> GTQQK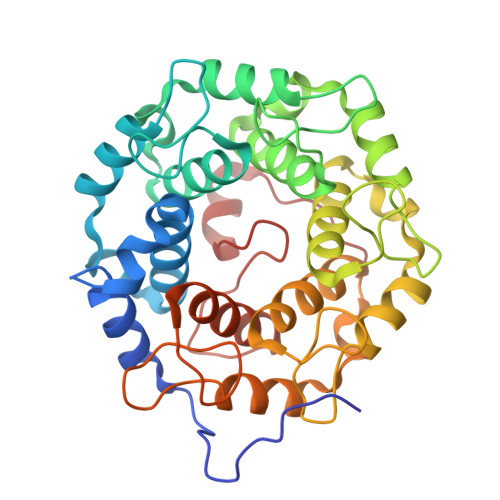DVTIKSDAPDTLLLEKHADYIASYGSKKDDYEYCMSEYLRMSGVYWGLTVMDLMGQLHRMNKEEILVFIKSCQHECGGVSASIGHDPHLLYTLSAVQILTLYDSIHVINVDKVVAYVQSLQKEDGSFAGDIWGEIDTRFSFCAVATLALLGKLDAINVEKAIEFVLSCMNFDGGFGCRPGSESHAGQIYCCTGFLAITSQLHQVNSDLLGWWLCERQLPSGGLNGRPEKLPDVCYSWWVLASLKIIGRLHWIDREKLRSFILACQDEETGGFADRPGDMVDPFHTLFGIAGLSLLGEEQIKPVSPVFCMPEEVLQRVNVQPELVS> KETAAAKFERQHMDSSTSAASSSNYCNQMMKSRNLTKDRCKPVNTFVHESLADVQAVCSQKNVACKNGQTNCYQSYSTMSITDCRETGSSKYPNCAYKTTQAN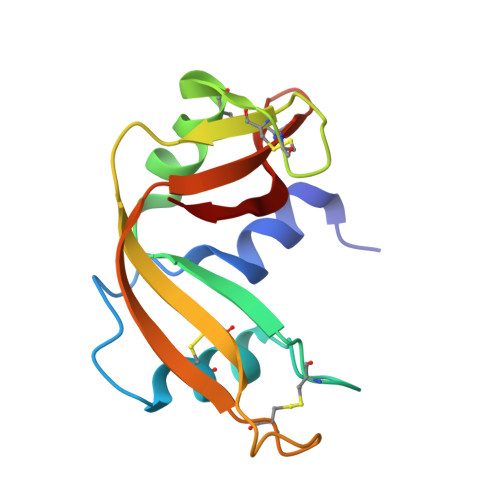KHIIVACEGNPYVPVHADASV>[4x]PTMTARQRVWRAFENPHTSTMALVFYYVTGFFIAVSVIANVVETVPCGSSPGHIKELPCGERYAVAFFCLDTACVMIFTVEYLLRLAAAPSRYRFVRSVMSIIDVVAILPYYIGLVMTDNEDVSGAFVTLRVFRVFRIFKFSRHSQGLRILGYTLKSCASELGFLLFSLTMAIIIFATVMFYAEKGSSASKFTSIPAAFWYTIVTMTTLGYGDMVPKTIAGKIFGSICSLSGVLVIALPVPVIVSNFSRIYHQNQ

Modulation of voltage-gated potassium (Kv) channels by auxiliary subunits is central to the physiological function of channels in the brain and heart. Native Kv4 tetrameric channels form macromolecular ternary complexes with two auxiliary β-subunits—intracellular Kv channel-interacting proteins (KChIPs) and transmembrane dipeptidyl peptidase-related proteins (DPPs)—to evoke rapidly activating and inactivating A-type currents, which prevent the backpropagation of action potentials. Here we report cryo-electron microscopy structures of the Kv4.2–DPP6S–KChIP1 dodecamer complex, the Kv4.2–KChIP1 and Kv4.2–DPP6S octamer complexes, and Kv4.2 alone. Thus, our data suggest that two distinct modes of modulation contribute in an additive manner to evoke A-type currents from the native Kv4 macromolecular complex.

The fourfold symmetrical structures of both Kv4.2 alone and the Kv4.2–KChIP1 complex were determined to an overall resolution of 2.9 Å by single-particle cryo-EM analysis with C4 symmetry imposed. The transmembrane domain of Kv4.2 adopts the Shaker-type topology, with the S1–S4 voltage-sensing domain and the S5–S6 channel pore forming helices composing a homo-tetramer in a domain-swapped manner, whereby the S1–S4 voltage sensor interacts with S5 of the pore domain from the neighbouring subunit. It adopts a depolarized S4 up and S6 open conformation in both Kv4.2 alone and Kv4.2–KChIP1. The C-terminal intracellular S6 helix continuously extends from the transmembrane S6 helix toward KChIP1, which was not observed in previous studies. In addition, the intracellular S6 helix interacts with the T1–S1 linker in the structure of the Kv4.2–KChIP1 complex. In addition, the open conformation of Kv4.2 complexes revealed several Kv4-specific residues involved in the intra-subunit interactions between the S4–S5 linker and S6, as well as the inter-subunit interactions between the S4–S5 linker and S5.>[10x]MSALLILALVGAAVADYKDDDDKLHSQANLMRLKSDLFNRSPMYP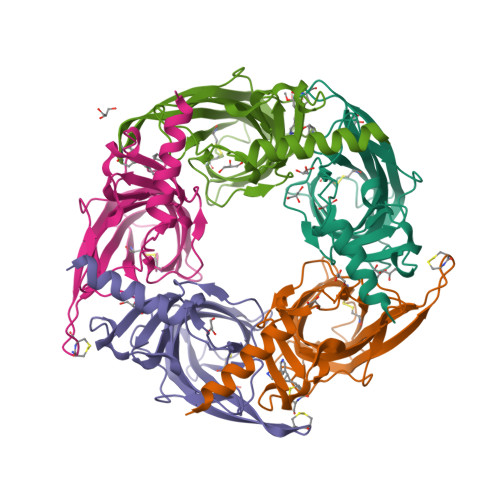GPTKDDPLTVTLGFTLQDIVKADSSTNEVDLVYYEQQRWKLNSLMWDPNEYGNITDFRTSAADIWTPDITAYSSTRPVQVLSPQIAVVTHDGSVMFIPAQRLSFMCDPTGVDSEEGATCAVKFGSWVYSGFEIDLKTDTDQVDLSSYYASSKYEILSATQTRQVQHYSCCPEPYIDVNLVVKFRERR HMPV (Paramyxoviridae, subfamily Pneumovirinae) is a leading cause of serious respiratory tract infections in children, the elderly, and immunocompromised individuals. In all members of the Mononegavirales, the RNA genome is packaged in the form of a nucleocapsid, a ribonucleoprotein complex consisting of polymerized viral nucleoproteins (N) and RNA. Besides protecting the viral genome from host nucleases, the nucleocapsid serves as the template for transcription by the viral RNA-dependent RNA polymerase L. Nucleocapsid assembly necessitates a pool of monomeric, RNA-free N, termed N0, which is kept in an unassembled state through an interaction with an N-terminal portion of the polymerase cofactor P, until delivered to the sites of viral RNA synthesis. In conclusion, the reported structures of a paramyxoviral N protein reveal two distinct conformational states, N bound either to the polymerase cofactor P or to RNA.

To this end, we purified and crystallized assembled HMPV N in the form of a decameric N-RNA ring. By exploiting the ten-fold non-crystallographic symmetry in the rings, we were able to obtain excellent electron density maps at 4.2-Å resolution and build a reliable model. Assembled HMPV decameric N-RNA rings are ~0.5 MDa in molecular mass and 160 Å in diameter and 70 Å in height. The observed RNA binding mode is similar to that seen in the related RSV N-RNA structure. The RNA wraps around the N ring and wedges tightly in the cleft between the NTD and CTD of N, which is lined by positively charged residues. Similar to N proteins from other members of Mononegavirales, the NTD- and CTD-arms grasp the neighbouring protomers, thus facilitating assembly of polymeric N. The NTD-arm packs against the flank of the previous protomer (the NTD-arm of Ni+1 packs against Ni). The CTD-arm in turn latches onto the top of the CTD of the next protomer (CTD-arm of Ni-1 latches onto CTD of Ni). Upon RNA binding, Thr257 contacts the backbone of a nucleotide instead of stabilizing Ala254. In the assembled, RNA-bound state these interactions are broken, with Arg186 and Trp261 now positioning RNA nucleotides in the cleft, whilst Arg260 instead fastens onto the NTD-arm of the neighbouring Ni+1.

>[10x]MSLQGIHLSDLSYKHAILKESQYTIKRDVGTTTAVTPSSLQQEITLLCGEILYAKHADYKYAAEIGIQYISTALGSERVQQILRNSGSEVQVVLTRTYSLGKIKNNKGEDLQMLDIHGVEKSWVEEIDKEARKTMATLLKESSGNIPQNQRPSAPDTPIILLCVGALIFTKLASTIEVGLETTVRRANRVLSDALKRYPRMDIPKIARSFYDLFEQKVYHRSLFIEYGKALGSSSTGSKAESLFVNIFMQAYGAGQTMLRWGVIARSSNNIMLGHVSVQAELKQVTEVYDLVREMGPESGLLHLRQSPKAGLLSLANCPNFASVVLGNASGLGIIGMYRGRVPNTELFSAAESYAKSLKESNKINFSSLGLTDEEKEAAEHFLNVSDDSQNDYEKHHHHHH>MAHTGRMFKIEAAEIVVARLPLKFRFETSFGVQTHKVVPLLILHGEGVQGVAEGTMEARPMYREETIAGALDLLRGTFLPAILGQTFANPEAVSDALGSYRGNRMARAMVEMAAWDLWARTLGVPLGTLLGGHKEQVEVGVSLGIQADEQATVDLVRRHVEQGYRRIKLKIKPGWDVQPVRATREAFPDIRLTVDANSAYTLADAGRLRQLDEYDLTYIEQPLAWDDLVDHAELARRIRTPLCLDESVASASDARKALALGAGGVINLKVARVGGHAESRRVHDVAQSFGAPVWCGGMLESGIGRA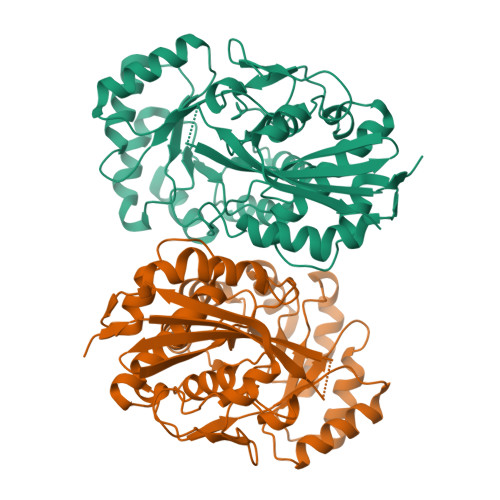HNIHLSTLSNFRLPGDTSSASRYWERDLIQEPLEAVDGLMPVPQGPGTGVTLDREFLATVTEAQEEHRA[4x]>[2x]EGDIHMKKGHHHHHHENLYFQGGSGKLSEQLKHCNGILKELLSKKHAAYAWPFYKPVDASALGLHDYHDIIKHPMDLSTVKRKMENRDYRDAQEFAADVRLM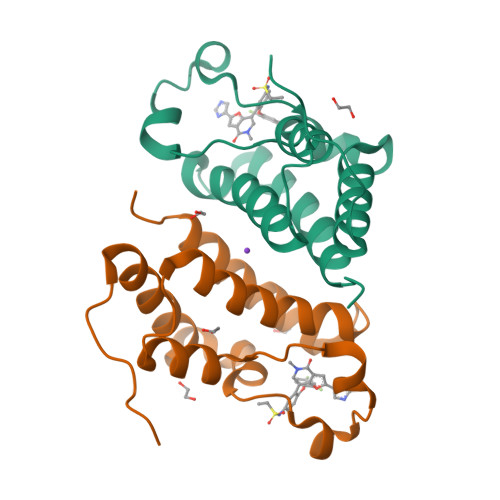FSNCYKYNPPDHDVVAMARKLQDVFEFRYAKMPD Escherichia coli NfsB has been studied extensively for its potential for cancer gene therapy by reducing the prodrug CB1954 to a cytotoxic derivative. The natural substrate of this flavoprotein enzyme is not known; however, it reduces a wide range of nitroaromatic compounds to hydroxylamines and also reduces quinones to quinols, with a bi-bi substituted (ping-pong) enzyme mechanism. The enzyme is a homodimer of two 24 kDa subunits with an extensive dimer interface. The two active sites are on opposite sides of the long central helix at the dimer interface, and the FMN is bound to residues from both monomers.

The most active mutant selected was T41Q/N71S/F124T. While the N71S is the only mutation at position 71 that enhances the activity of the protein for CB1954, the F124T mutation is not the most active mutation at position 124, and the T41Q mutation by itself reduces the activity of the protein for CB1954. The mutations together, therefore, show synergistic effects. In this study, structures of the double and triple mutant were both determined with and without bound nicotinic acid. In the triple mutant, the N71S mutation is the same as in the double mutant; position 41, however, is now a Gln, which is larger than the wild-type threonine and more polar than the leucine of the double mutant, while F124 has been replaced by threonine. In the structures of the free and nicotinate-bound triple mutant, the Q41 side chain forms a hydrogen bond to the T124 hydroxyl group, pulling the residue slightly closer than in the wild-type protein. In the structure with bound nicotinate, the Q41 side chain interacts with the nicotinate ring and is in a different orientation to the side chain of the L41 mutant. In the structures of the proteins bound to nicotinate, both L41 and Q41 interact with the nicotinamide ring and are likely to also interact with CB1954. The crystal structure of the T41Q/N71S/F124T mutant shows a hydrogen bond between Q41 and T124, explaining the co-operativity between these two residues. On replacing N71 with S71, in most of the structures of all the mutants, a water-mediated hydrogen bond to the FMN cofactor is found from the Oγ of S71 instead of the direct hydrogen bond from the NH2 of N71.

>[2x]DIISVALKRHSTKAFDASKKLTPEQAEQIKTLLQYSPSSQNSQPWHFIVASTEEGKARVAKSAAGNYVFSERKMLDASHVVVFCAKTAMDDVWLKLVVDQEDADGRFATPEAKAANDKGRKFTADMHRKDLHDDAEWMAKQVYLNVGNFLLGVAALGLDAVPIEGFDAAILDAEFGLKEKGYTSLVVVPVGHHSVEDFNATLPKSRLPQNITLTEV> M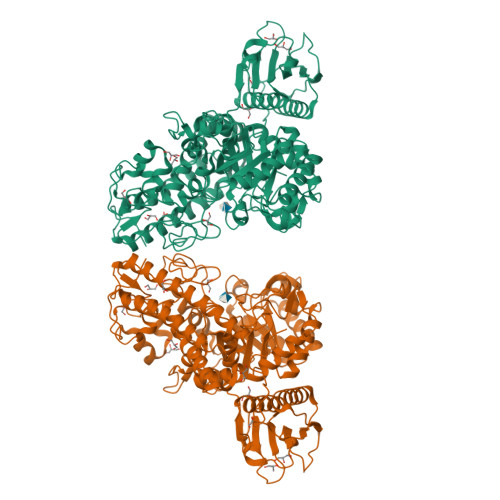TAGYEPCWLRYERKDQYSRLRFEEIVAKRTSPIFQAAVEELQKGLRSMMEIEPQVVQEVNETANSIWLGTLEDEEFERPLEGTLVHPEGYVIRSDVDDGPFRIYIIGKTDAGVLYGVFHFLRLLQMGENIAQLSIIEQPKNRLRMINHWDNMDGSIERGYAGRSIFFVDDQFVKQNQRIKDYARLLASVGINAISINNVNVHKTETKLITDHFLPDVAEVADIFRTYGIKTFLSINYASPIEIGGLPTADPLDPEVRWWWKETAKRIYQYIPDFGGFVVKADSEFRPGPFTYGRDHAEGANMLAEALAPFGGLVIWRCFVYNCQQDWRDRTTDRAKAAYDHFKPLDGQFRENVILQIKNGPMDFQVREPVSPLFGAMPKTNQMMEVQITQEYTGQQKHLCFLIPQWKEVLDFDTYAKGKGSEVKKVIDGSLFDYRYSGIAGVSNIGSDPNWTGHTLAQANLYGFGRLAWNPDLSAEEIANEWVVQTFGDDSQVVETISWMLLSSWRIYENYTSPLGVGWMVNPGHHYGPNVDGYEYSHWGTYHYADRDGIGVDRTVATGTGYTAQYFPENAAMYESLDTCPDELLLFFHHVPYTHRLHSGETVIQHIYNTHFEGVEQAKQLRKRWEQLKGKIDEKRYHDVLERLTIQVEHAKEWRDVINTYFYRKSGIDDQYGRKIYR>MGSSHHHHHHMTLNQPEYFTKYENLHFHRDENGILEVRMHTNGSSLVFTGKTHREFPDAFYDISRDRDNRVVILTGSGDAWMAEIDFPSLGDVTNPREWDKTYWEGKKVLQNLLDIEVPVISAVNGAALLHSEYILTTDIILASENTVFQDMPHLNAGIVPGDGVHILWPLALGL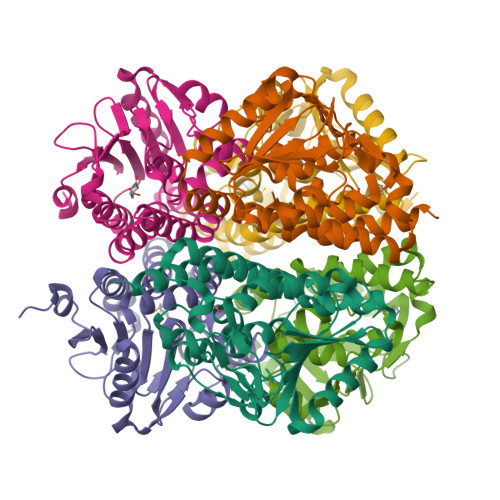YRGRYFLFTQEKLTAQQAYELNVVHEVLPQSKLMERAWEIARTLAKQPTLNLRYTRVALTQRLKRLVNEGIGYGLALEGITATDLRNT[2x]>[2x]SRKTYTLTDYLKNTYRLKLYSLRWISDHEYLYKQENNILVFNAEYGNSSVFLENSTFDEFGHSINDYSISPDGQFILLEYNYVKQWRHSYTASYDIYDLNKRQLITEERIPNNTQWVTWSPVGHKLAYVWNNDIYVKIEPNLPSYRITWTGKEDIIYNGITDWVYEEEVFSAYSALWWSPNGTFLAYAQFNDTEVPLIEYSFYSDESLQYP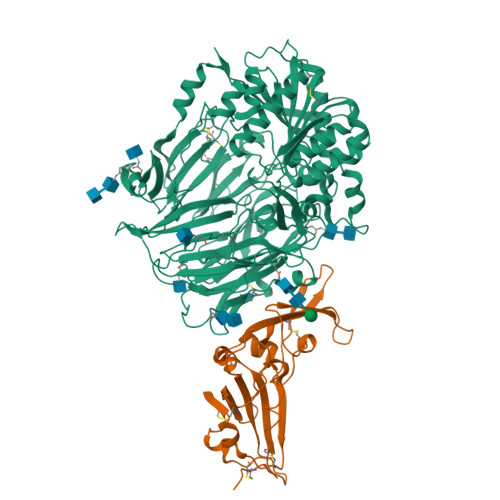KTVRVPYPKAGAVNPTVKFFVVNTDSLSSVTNATSIQITAPASMLIGDHYLCDVTWATQERISLQWLRRIQNYSVMDICDYDESSGRWNCLVARQHIEMSTTGWVGRFRPSEPHFTLDGNSFYKIISNEEGYRHICYFQIDKKDCTFITKGTWEVIGIEALTSDYLYYISNEYKGMPGGRNLYKIQLSDYTKVTCLSCELNPERCQYYSVSFSKEAKYYQLRCSGPGLPLYTLHSSVNDKGLRVLEDNSALDKMLQNVQMPSKKLDFIILNETKFWYQMILPPHFDKSKKYPLLLDVYAGPCSQKADTVFRLNWATYLASTENIIVASFDGRGSGYQGDKIMHAINRRLGTFEVEDQIEAARQFSKMGFVDNKRIAIWGWSYGGYVTSMVLGSGSGVFKCGIAVAPVSRWEYYDSVYTERYMGLPTPEDNLDHYRNSTVMSRAENFKQVEYLLIHGTADDNVHFQQSAQISKALVDVGVDFQAMWYTDEDHGIASSTAHQHIYTHMSHFIKQCFSLPHHHHHH;>[2x]EASATGTFIEQPNATECDFSPMLTGVAPQVYNFKRLVFSNCNYNLTKLLSLFAVDEFSCNGISPDSIARGCYSTLTVDYFAYPLSMKSYIRPGSAGNIPLYNYKQSFANPTCRVMASVLANVTITKPHAYGYISKCSRLTGANQDVETPLYINPGEYSICRDFSPGGFSEDGQVFKRTLTQFEGGGLLIGVGTRVPMTDNLQMSFIISVQYGTGTDSVCPMLDLGDSLTITNRLGKCVDYHHHHHH> GTHSLKYVYTGVSRGIDFPEFTAVGMVDDGQFMYFDSNSMKAVPKTEWIRQNEGADYWDRQTQVLIGAHQVFKDSIQIVMERFNQSKGVHTWQNMYGCELNDDGTTQGFYQYAYDGEDFVSLDKNTLTWTAANPQAVITKHKWEALAVAEQNKGYLENTCIEWLKKYVAYGKDTLERKVSPQVSLLQKDPSSPVTCHATGFYPSGVTI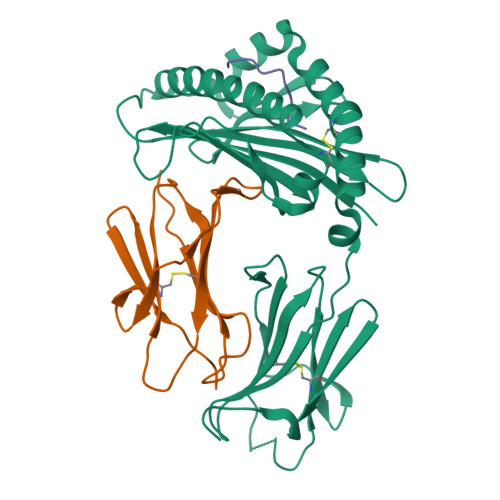TWQKNGQDHDEDVDLGELLPNEDGSFQRMSTLNVGPDEWKNNRFSCVVEHQDKTIRKTEDDIITNFD;> MRALVSFALFCVLYISVQGKVSSPKIQVYSHYPGEYGKENTLICYVSGFHPPDISIELLKNGEVIADAQQTDLAFEKGWQFHLTKSVSFKPEKSDEYSCSVRHMSKTKKIVWESNM;> FANFCLMMI> SMGVRKLATIRTAGEITPIAGAEAIECCHVDGWTCVIKKGEFKQGDRGVYFEIDSFIKEDNDRYPMLSKQVIDYEGQRGTRLRTARLRGQLSQGLFLPMDRFPELASNQVGDDVTEILGITKWEPPISTNLSGEILGEFPTFISKTDQERVQNLIPQIEENKGQKFEVTVMLDGSSMTVYRKDDHIGVCGRNWELRETATNAQWHAARRNKMIEGLQFLNRNLALQGEIIGESIQGNLEKLKGQDFYLFDIYDIDKAQYLTPIERQSLVKQLNDNGFTVKHVPILDDLELNHTAEQILAMADGPSLNKNVKREGLVFKRLDGKFSFKAI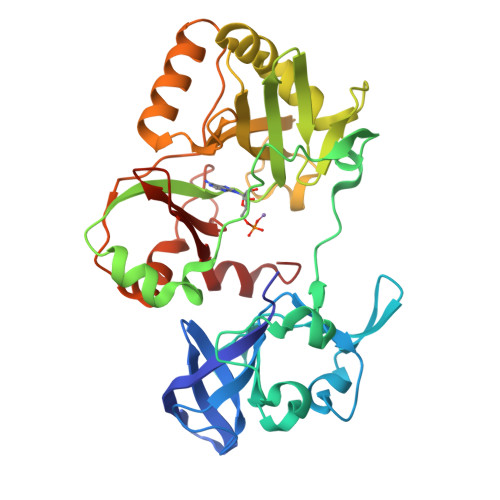SNAYLEKHKDR>MILVTG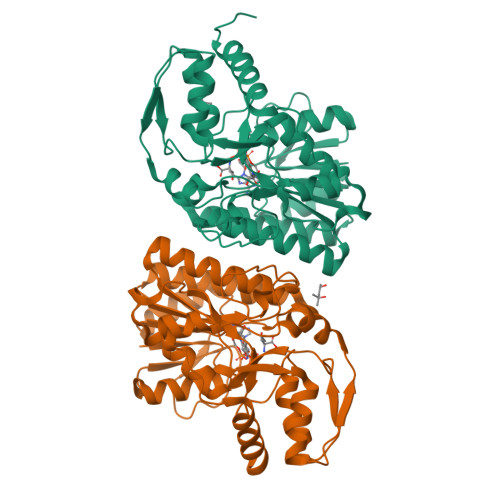SSGQIGTELVPYLAEKYGKKNVIASDIVQRDTGGIKFITLDVSNRDEIDRAVEKYSIDAIFHLAGILSAKGEKDPALAYKVNMNGTYNILEAAKQHRVEKVVIPSTIGVFGPETPKNKVPSITITRPRTMFGVTKIAAELLGQYYYEKFGLDVRSLRYPGIISYKAEPTAGTTDYAVEIFYYAVKREKYKCYLAPNRALPMMYMPDALKALVDLYEADRDKLVLRNGYNVTAYTFTPSELYSKIKERIPEFEIEYKEDFRDKIAATWPESLDSSEASNEWGFSIEYDLDRTIDDMIDHISEKLGIEGKHAL[2x]7-[({2-[4-(dimethylamino)phenyl]ethyl}amino)methyl]quinolin-2-amine | C20 H24 N4 | 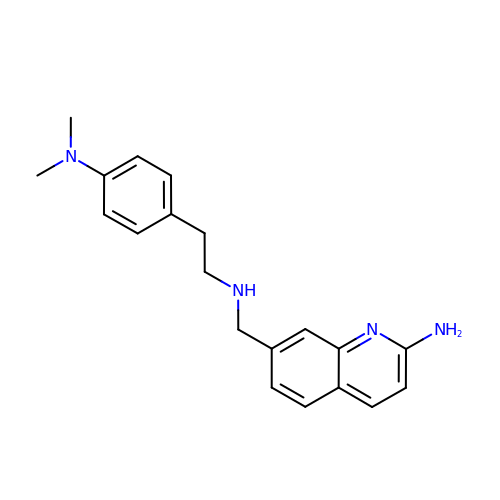SYHMYZCWRIEYOI-UHFFFAOYSA-N>[2x]MSLGELNVATVTRRPEILLVDS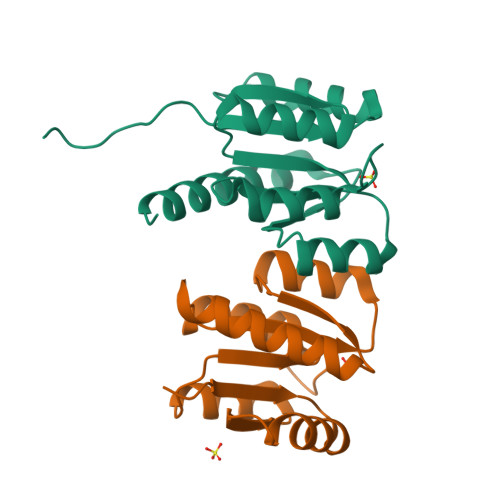QEVILQRLQQLLSPLPYTLHFARDATQALQLLASREVDLVISAAHLPQMDGPTLLARIHQQYPSTTRILLTGDPDLKLIAKAINEGEIYRYLSKPWDDQELLLALRQALEHQHSERERLRLQDEGHHHHHH> IDPFTAKRTHRVINHPYYFPFNGRQAEDYLRSKERGEFVIRQSSRGDDHLVITWKLDKDLFQHIDIQELEKENPLALGKVLIVDNQKYNDLDQIIVEYLQNKVRLLNEMTSSEKFKSGTKKDVVKFIEDYSRVNPNKSVYYFSLNHDNPGWFYLMFKINANSKLYT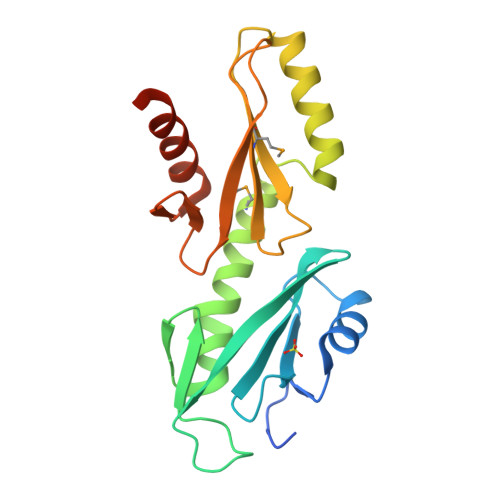WNVKLTNTGYFLVNYNYPSVIQLCNGFKTLLKSNSSKNRMNNYR> SMMKRVHRTDVKAEIVREPGAKETTHRKLIDTPDGADRFVLTEFEVSPNGSTPPHFHEWEHEIYVLE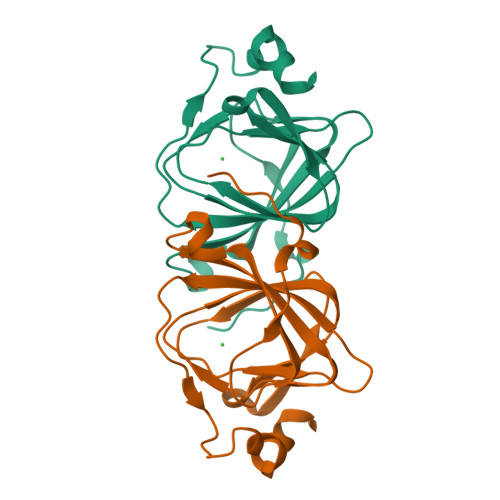GSMGLVLPDQGRTEEVGPGEAIFIPRGEPHGFVTGPGQTCRFLVVAPCERPPVRNVFLSEDPYEYTQMPEYTSLLESK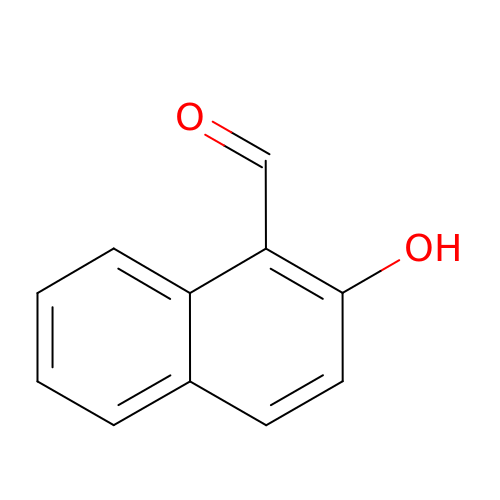2-hydroxynaphthalene-1-carbaldehyde | C11 H8 O2 | NTCCNERMXRIPTR-UHFFFAOYSA-N> MSDIFNSPQNKASILTALMKSTTGDVEDVLIPKRFRPAKDPLDSPQAAAQFLKDNKYRILRPRAIPTMVELETDAALPRLRQMVEDGKLKDTVSVPEGTTAFYPKYYPFHKPDHDEVGTFGAPDITLLKQLTFFLLENDFPTGPETLRQVREAIATLQYGSGSYSGQLNRLLAMKGVATGRNPNKTPKTVGYTNEQLAKLLEQTLPINTPKHEDPDLRWAPSWLINYTGDLSTDKSYLPHVTIKSSAGLPYIGKTKGDTTAEALVLADSFIRDLGRAATSADPEAGVKKTITDFWYLSCGLLFPKGERYTQVDWDKKTRNIWSAPYPTHLLLSMVSTPVMNESKLNITNTQTPS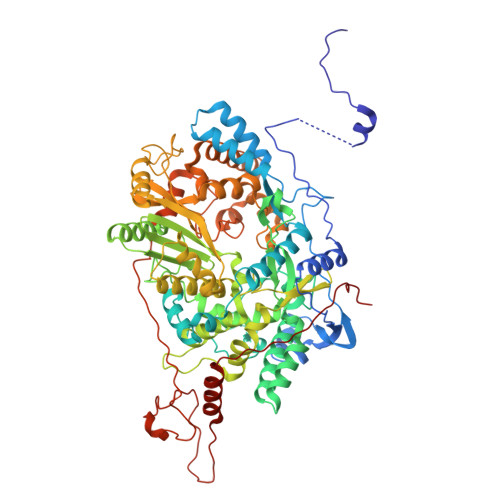LYGFSPFHGGMDRIMTIIRDSLDNDEDLVMIYADNIYILQDNTWYSIDLEKGEANCTPQHMQAMMYYLLTRGWTNEDGSPRYNPTWATFAMNVAPSMVVDSSCLLMNLQLKTYGQGSGNAFTFLNNHLMSTIVVAEWVKAGKPNPMTKEFMDLEEKTGINFKIERELKNLRETIVEAVETAPQDGYLADGSDLPPIRPGKAVELDLLGWSAIYSRQMEMFVPVLENERLIASAAYPKGLENKALARKPGAEIAYQIVRYEAIRLVGGWNNPLLETAAKHMSLDKRKRLEVKGIDVTGFLDDWNNMSEFGGDLEGITLSEPLTNQTLVDINTPLXXXXXXXXXXXXXXXXXXXXXXXXXXXXXXXXXXXXXXXXXXXXXXXXXXXXXXXXXXXXXXXXXXXXXXXXXXXXXXXXXXX> SLRYSRHDGTSCVIDNHHLKSLGAVLNDVRRKKDRIREAEYEPIIDIADQYMVTEDPFRGPGKNVRITLFKEIRRVHPDTMKLVCNWSGKEFLRETWTRFISEEFPITTDQEIMDLWFELQLRPMHPNRCYKFTMQYALGAHPDYVAHDVIRQQDPYYVGPNNIERINLSKKGFAFPLTCLQSVYNDNFERFFDDVLWPYFYRPLVYVGTTSAEIEEIMIEVSLLFKIKEFAPDVPLFTGPAY

Using pulses from X-ray free-electron lasers (XFEL) with sufficiently short duration to outrun radiation damage, the structures of biological macromolecules can be obtained from nanocrystals at room temperature12. The resulting method is referred to as serial femtosecond crystallography (SFX)2. In the double-flow focusing nozzle (DFFN) that we present here, an inner liquid jet is focused by a coaxial faster outer liquid jet that is itself focused by gas as in the traditional GDVN. Our DFFN system reduces sample consumption up to eight fold compared to a GDVN, can inject crystals in their native crystallization buffers, and is suitable for time-resolved mixing experiments and future high repetition rate X-ray sources such as LCLS-II.

Because of the low X-ray background and focusing of the sample, DFFN injection is also well suited for diffraction data collection of very small crystals. Cydia pomonella granulovirus (CpGV) crystals are the smallest crystals used so far for structure determination by SFX15, with an average size of 400 × 200 × 200 nm3 (and about 10,000 unit cells per crystal). Using CpGV, we further analyzed how the fraction of pulses, which show crystal diffraction (the “hit fraction”), depends on the sample flow rate and the type of sheath liquid, for a given crystal concentration. The average hit fractions of 8–10% obtained at these low sample flow rates indicates the continuous operation of a stable jet over the course of the experiment and the absence of interruptions that often accompany experiments that use GVDNs. Even so, either the use of water or ethanol as sheath liquids leads to stable jets at much reduced sample flow-rates as compared to normal GDVN injection.> SPSSELRRALEANEFIPYYQPLSPGQGGRWIGVEVLMRWRHPREGLIRPDLFIPFAERSGLIVPMTRALMRQVAEDLGGHAGKLEPGFHIGFNISATHCHELALVDDCRELLAAFPPGHITLVLELTERELIESSEVTDRLFDELHALGVKIAIDDFGTGHSSLAYLRKFQVDC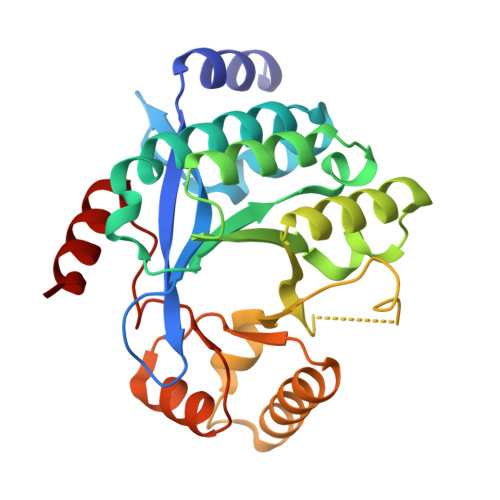LKIDQSFVARIGIDTLSGHILDSIVELSAKLDLDIVAEGVETPEQRDYLAARGVDYLQGYLIGRPMPLESLLSSLTVQEG4-{2-[(6-amino-8-oxo-7,8-dihydro-1H-imidazo[4,5-g]quinazolin-2-yl)amino]ethyl}benzoic acid | C18 H16 N6 O3 | 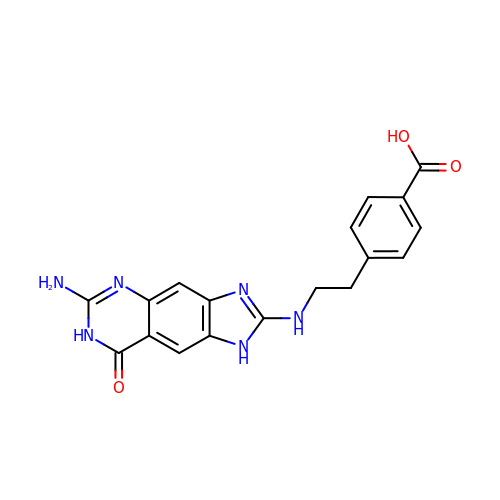TZNQMGFEWYPGDR-UHFFFAOYSA-N> MTHLERSRHQQHPFHMVMPSPWPIVVSFALLSLALSTALTMHGYIGNMNMVYLALFVLLTSSILWFRDIVAEATYLGDHTMAVRKGINLGFLMFVLSEVLIFAGLFWAYFHSAMSPDVTLGACWPPVG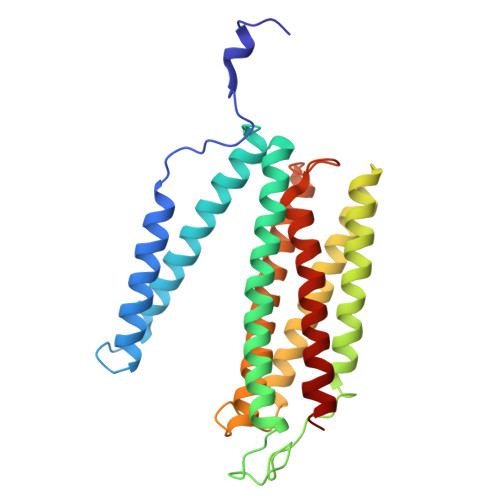IEAVQPTELPLLNTIILLSSGATVTYSHHALIAGNRNKALSGLLITFWLIVIFVTCQYIEYTNAAFTISDGVYGSVFYAGTGLHFLHMVMLAAMLGVNYWRMRNYHLTAGHHVGYETTIIYTHVLDVIWLFLYVVFYWWGV> MVSVANAAQTPAAQETTKNVTIMHISTIYDKTGKATNEPALRAYDTVSVVSDP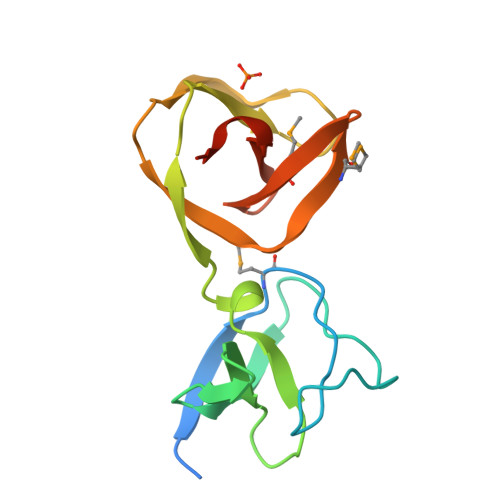VTINNAKFYKLAGKDQYIKVGNVDGTSRTLKHNSYVYKSSGKRANKKTLKKGSSVTTYGKSFMIAGHQMYRIGKNQYVKKANFLEHHHHHH>MSLEVYVLRLGHRPERDKRISTHVALTARAFGAKGIYFDTEDKSVFESVRDVVERWGGDFFIKAVSWKKLLREFDGLKV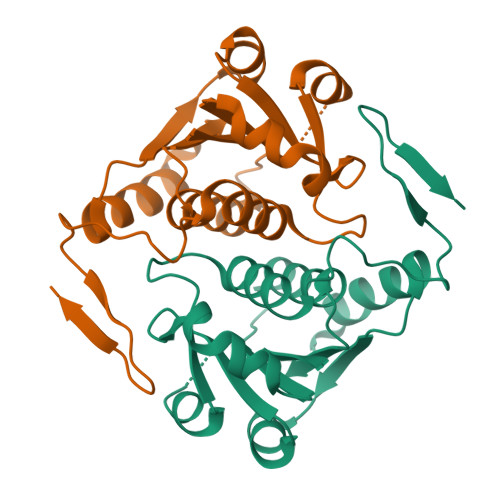HLTMYGIPLPQKLEEIKRADKVLVVVGAEKVPPEVYELCDLNISIGTQPHSEVAALAVFLDRVLGKVFDISFDDAKIKVIPSERGKRVVSEEGHHHHHH[2x]>MATLKDIGVSAGINILTAFIFFIIFAFLRLQPFNDRVYFSKWYLRGLRSSPASGGGFAGRFVNLELRSYLKFLHWMPEALKMPERELIDHAGLDSVVYLRIYWLGLKIFAPIAMLAWAVLVPVNWTNNELELAKHFKNVTSSDIDKLTISNIPEGSNRFWAHIIMAYAFTIWTCYMLMKEYETVANMRLQFLASEGRRPDQFTVLVRNVPPDPDETVSELVEHFFLVNHPDNYLTHQVVCNANKLADLVSKKTKLQNWLDYYQLKYTRNNSQIRPITKLGCLGLCGQKVDAIEHYIAEVDKTSKEIAEERENVVNDQKSVMPASFVSFKTRWAAAVCAQTTQTRNPTEWLTEWAAEPRDIYWPNLAIPYVSLTVRRLVMNVAFFFLTFFFIIPIAFVQSLATIEGIEKVAPFLKVIIEKDFIKSLIQGLLAGIALKLFLIFLPAILMTMSKFEGFTSVSFLERRSASRYYIFNLVNVFLGSVIAGAAFEQLNSFLNQSPNQIPKTIGMAIPMKATFFITYIMVDGWAGVAGEILMLKPLIIYHLKNAFLVKTEKDREEAMNPGSIGFNTGEPQIQLYFLLGLVYAPVTPMLLPFILVFFALAYVVYRHQIINVYNQEYESAAAFWPDVHGRVITALIISQLLLMGLLGTKHAASAAPFLIALPVITIGFHRFCKGRFEPAFVRYPLQEAMMKDTLERAREPNLNLKGYLQDAYIHPVFKGGDNDDDGDMIGKLENEVIIVPTKRQSRRNTPAPSR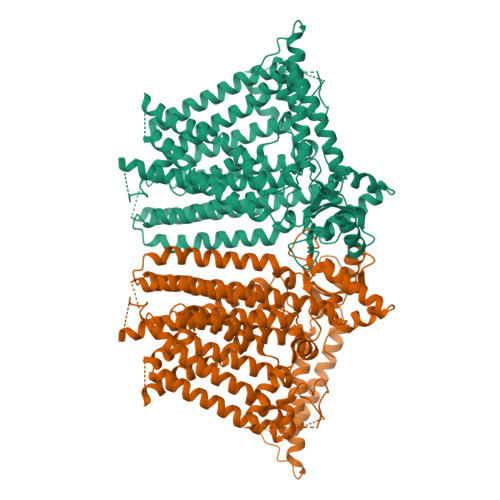ISGESSPSLAVINGKEV[2x]> MGIQGLAKLIADVAPSAIRENDIKSYFGRKVAIDASMSIYQFLIAVRQGGDVLQNEEGETTSHLMGMFYRTIRMMENGIKPVYVFDGKPPQLKSGELAKRSERRAEAEKQLQQAQAAGAEQEVEKFTKRLVKVTKQHNDECKHLLSLMGIPYLDAPSEAEASCAALVKAGKVYAAATEDMDCLTFGSPVLMRHLTASEAKKLPIQEFHLSRILQELGLNQEQFVDLCILLGSDYCESIRGIGPKRAVDLIQKHKSIEEIVRRLDPNKYPVPENWLHKEAHQLFLEPEVLDPESVELKWSEPNEEELIKFMCGEKQFSEERIRSGVKRLS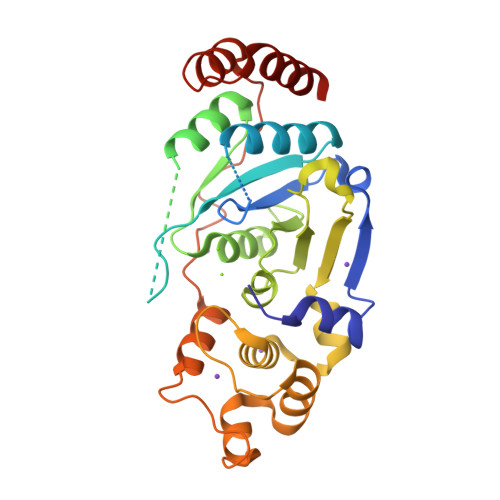KSRQ> MADEIAKAQVARPGGDTIFGKIIRKEIPAKIIFEDDQALAFHDISP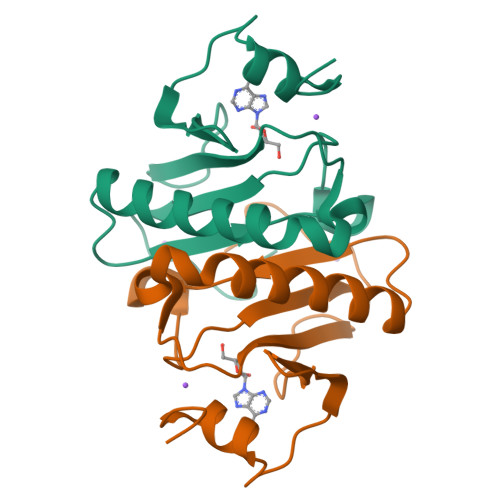QAPTHFLVIPKKHISQISAAEDADESLLGHLMIVGKKCAADLGLKKGYRMVVNEGSDGGQSVYHVHLHVLGGRQMNWPPG>[6x]GASGDLYEVERIVDKR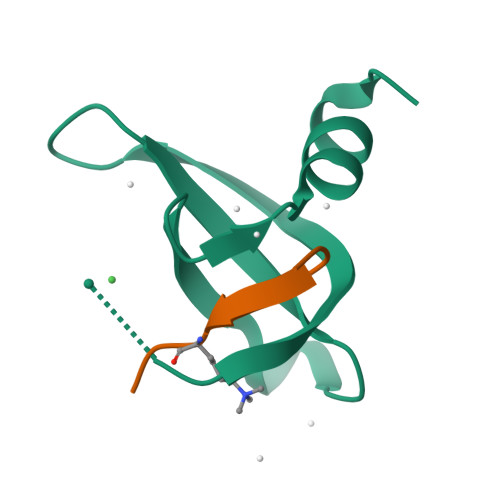KNKKGKWEYLIRWKGYGSTEDTWEPEHHLLHCEEFIDEFNGLHMSK;>[6x]XATKVARKSAPATX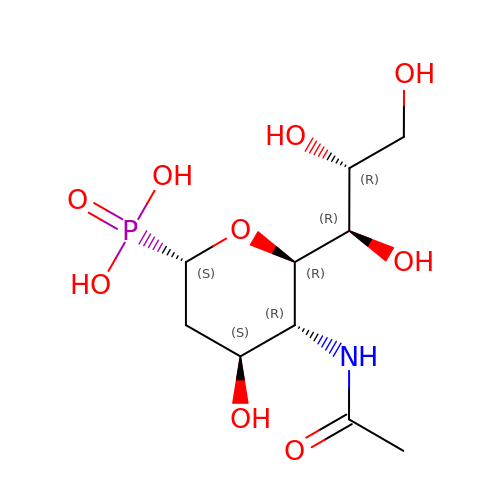(1S)-4-acetamido-1,5-anhydro-2,4-dideoxy-1-phosphono-D-glycero-D-galacto-octitol | C10 H20 N O9 P | QITAGYVZDNZULE-HDBWYCHPSA-N>MVALKGIPKVLSPELLFALARMGHGDEIVLADANFPTSSICQCGPVEIRADGLDIPQLLEAVLRLLPLDTYVESPAAVMDLVPSDKEKGLQTPIWKRYESLLLEADCKKTLMKLERFEFYERAKKAFAVVATGEMALYGNIILK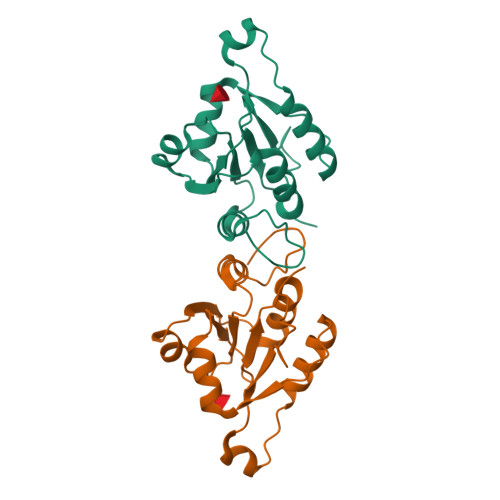KGTLD[2x]> ILVPMTVNDQPIEKNGDKMPLKFKLGPLSYQNMAFITAKDKYKLYPVRIPRLDTSKEFSAYVSGLFEIYRDLGDDRVFNVPTIGVVNSNFAKEHNATVNLAMEAILNELEVFIGRVKDQDGRVNRFYELEESLTVLNCLRTMYFILDGQDVEENRSEFIESLLNWINRSDGEPDEEYIEQVFSVKDSTAGKKVFET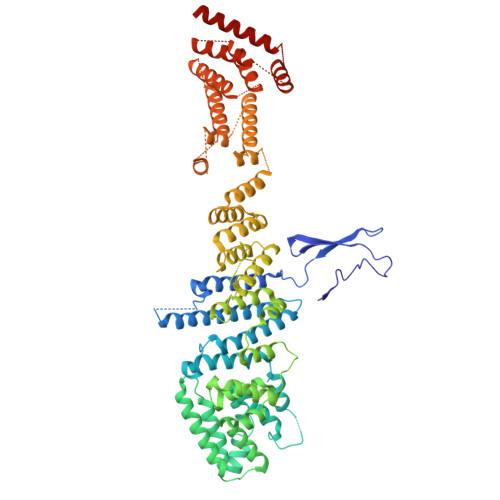QYFWKLLNQLVLRGLLSQAIGCIERSDLLPYLSDTCAVSFDAVSDSIELLKQYPKDSSSTFREWKNLVLKLSQAFGSSATDISGELRDYIEDFLLVIGGNQRKILQYSRTWYESFCGFLLYYIPSLELSAEYLQMSLEANVVDITNDWEQPCVDIISGKIHSILPVMESLDSCTAAFTAMICEAKGLIENIFEGEKNSDDYSNEDNEMLEDLFSYRNGMASYMLNSFAFELCSLGDKELWPVAIGLIALSATGTRSAKKMVIAELLPHYPFVTNDDIEWMLSICVEWRLPEIAKEIYTTLGNQMLSAHNIIESIANFSRAGKYELVKSYSWLLFEASCMEGQKLDDPVLNAIVSKNSPAEDDVIIPQDILDCVVTNSMRQTLAPYAVLSQFYELRDREDWGQALRLLLLLIEFPYLPKHYLVLLVAKFLYPIFLLDDKKLMDEDSVATVIEVIETKWDDADEKSSNLYETIIEADKSLPSSMATLLKNLRKKLNFKLCQAFM>MTQQITLIKDKILSDNYFTLHNITYDLTRKDGEVIRHKREVYDRGNGATILLYNTKKKTVVLIRQFRVATWVNGNESGQLIESCAGLLDNDEPEVCIRKAAIEETGYEVGEVRKLFELYMSPGGVTE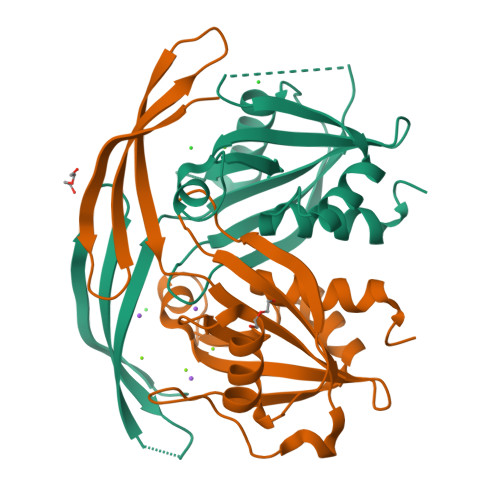LIHFFIAEYSDNQRANAGGGVEDEDIEVLELPFSQALEMIKTGEIRDGKTVLLLNYLQTSHLMD[2x]> GIPRRITKETQNLANEPPPGIMAVPVPENY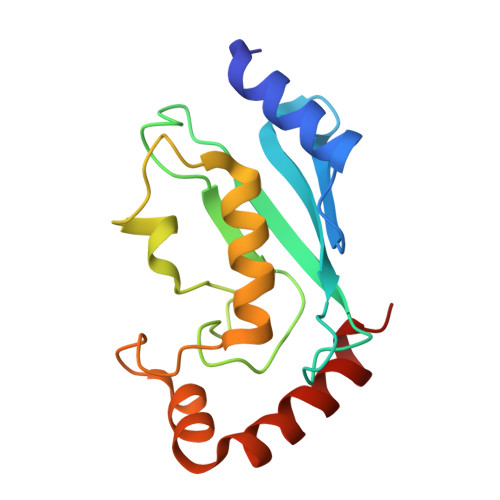RHFNILINGPDGTPYEGGTYKLELFLPEQYPMEPPKVRFLTKIYHPNIDKLGRICLDILKDKWSPALQIRTVLLSIQALLSSPEPDDPLDSKVAEHFKQDKNDAEHVARQWNKIYANNN The astacins are a family of metallopeptidases that share a central ∼200-residue catalytic domain (CD), which is found in >1000 species across holozoans and, sporadically, bacteria. Astacins share a basic domain architecture consisting of an N-terminal signal peptide for secretion, a pro-peptide (PP) of variable length (from 34 residues in astacin to 486 residues in Drosophila melanogaster tolkin; Finelli et al., 1995; Gomis-Rüth, Trillo-Muyo et al., 2012; Arolas et al., 2018) for zymogenic latency and the CD. The short paralogue has the basic domain architecture of the family, while the long paralogue further contains an LNK and an MAM domain. Here, we crystallized the zymogen of the long paralogue, hereafter referred to as pLAST-MAM, and solved its crystal structure.

After extensive calculations with the whole molecule and separate domains, the two CDs (N49–C244) could confidently be placed, rebuilt and refined, as well as the respective PPs (defined for E22–K48). In contrast, the LNK (F245–D257) and MAM (F258–C403) moieties were flexible and only those of protomer A could be placed in the structure. The intervening residues are included in a ‘PP motif’ found in astacins (F-E/Q-G-D-I; Gomis-Rüth, Trillo-Muyo et al., 2012), F35-E-G-D-I39 in pLAST. The primary activation site of pLAST (K48–N49) is inserted within short helix α2 and buried in the zymogen, thus preventing access by activating enzymes in a similar fashion as found in pro-astacin. Next, N49 would bind the ‘family-specific residue’ immediately after the third zinc-binding histidine (E150; Bode et al., 1993; Gomis-Rüth, 2003), which in turn is held in place by internal salt bridges with R237 and R153 in the zymogen.

>[2x]ENLGDLPLYHSNLFEGDIAGVSPYADKNAIVDHTLLWPGGIVYYELAPAAASIRNQILEGMKEYHEKTCIQFKERTAGVKDYIRINRYDGCWSMVGRQGGMQELSLGYGCEWKGLVVHALGHAVGFWHEQNRADRDDYIEVIWDNILQSMQYNFNKMEPWENNYLNERFDYKSVMLYGETAFSKDGTSPTVRPKQPGVVIGPVWKKPGFSESDVRRVNRLYECFGEVRPPPPKIPDFICDFESNDCGLENQVGMRGEFQRKYDTLGGRTGYFMVLSVTSSGTYADSRLITPYFGAYGNQDVCMSVDVYMSGPAVRDVEISRQDSNTESIGKYTEVSNSWVTRNFNLKAGREDMRFFIFAALDPYYGDGVVAVDNLKFKRKPC> GSNQNVKCKIVVVGDSQCG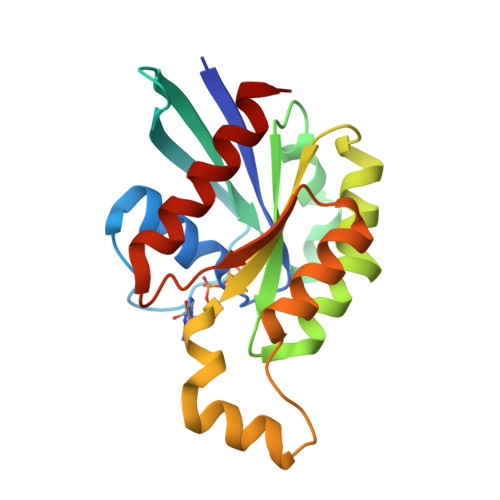KTALLHVFAKDCFPENYVPTVFENYTASFEIDTQRIELSLWDTSGSPYYDNVRPLSYPDSDAVLICFDISRPETLDSVLKKWKGEIQEFCPNTKMLLVGCKSDLRTDVSTLVELSNHRQTPVSYDQGANMAKQIGAATYIECSALQSENSVRDIFHVATLACVNK>GSHMEAVQNRIVEAAERVPGVRGVIHLRARYVGQDIWAAMIIGVDPENTVEQAHEICEAVQAAVCGKIRRIESLAVSAEAREIGDTTKPSFSDQPLSFDEVMLSKVDN[2x]

One group of metal ion efflux transporters that regulates metal ion homeostasis and can be found in all domains of life is the Cation Diffusion Facilitator (CDF) protein family. One of the most highly conserved and abundant integral MM proteins is the CDF transporter MamM. MamM was recently proposed to function as a magnetosome-directed iron transporter required for iron biomineralization since its deletion abolished magnetite biomineralization and mutation of residues within the conserved TMD metal-binding site resulted in alterations of magnetite crystal size, morphology and even mineral phase. To summarize our results we present an alternative model for the CDF CTD mode of action, in which we propose that upon metal cation binding, the CTD induces conformational changes towards a tighter and more compact fold which allows the activation of iron transport through the TMD.

To gain a better understanding of the contribution of these binding sites to protein function two double alanine point mutations were also analyzed. In vivo the introduction of double point mutations in the central putative binding site (D249A and H285A) resulted in decreased Cmag values similar to D249A. Although the average particle number per cell was almost identical between the D249A and the D249A + H285A strains, the latter strain produced particles with significantly reduced mean diameters (−12%, P<0.001, Mann-Whitney test). In addition, this strain also showed a slower restoration of its magnetic response upon induction of biomineralization by adding iron back to iron-starved cells. ITC results for the central putative binding site double mutant (D249A and H285A) displayed a reduced number of binding sites (1.8±0.2) in reference to the wild-type data and therefore suggests that a single cation binds to each peripheral binding site. To confirm that these observed phenotypic differences are due to true transport function alternations, we also examined the expression levels of all MamM mutants, their ability to stabilize MamB expression, performed MD simulations for dimer stability evaluation and determined their CTD structures. (ii) All mutants exhibited an apo-MamM CTD-like behavior along the MD simulations (see Fig. B in file S1 for representative MD simulations), and (iii) an absence of structural differences was observed.>LLPILSFPDPRLRTIAKPVEEVTDEIRQLAADMFETMYAAPGIGLAASQVDRHIQLIVMDLSESKDEPMVFINPKVTPLTEETQPYEEGCLSVPQIYDKVDRPSRVKIEAINLEGQAFEIEADGLLAVCIQ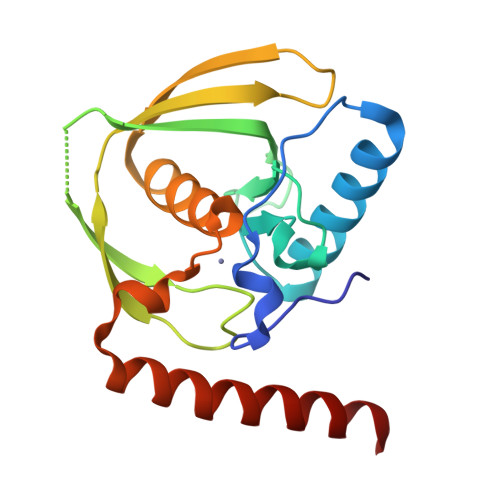HEMDHLNGKLFVDYLSPLKRQRAREKVEKIVRQREREKVA[2x]>MEHKYKNHLPKIHETTFVAEGVHIIGDVEIGEDSNIWFNAVLRGDVNSIKIGRGTNIQDNATLHASTGQSPTIIGDYVTVGHNCIIHGCKIGDYSLIGMGSIILDNAEIGEYTIIGAGSLVTQNKKIPPRVLCMGSPAKVIRELTEEEIEYLKNSAKHYIELSKNYRHHHHHH[3x]

The 16S microbial community profiling of a metagenomics library from geothermal spring at Lisvori (Lesvos island, Greece) enabled the identification of a putative sequence exhibiting 95% identity to the γ‐type carbonic anhydrase (γ‐CA) from Caloramator australicus (γ‐CaCA). The sequence of γ‐CaCA was amplified by PCR, cloned, and expressed in E. coli. X‐ray crystallographic analysis of the γ‐CaCAmut structure at 2.1 Å resolution, provided detailed structural insights into how the mutations impact the overall enzyme structure, function, and thermostability. These findings provide valuable structural and functional insights into γ‐CAs and demonstrate a strategy for converting an inactive enzyme into a catalytically active form through rational design.

Activity assays showed that γ‐CaCA possesses very low, but detectable, anhydrase activity, while exhibiting no measurable esterase activity. Differential scanning fluorimetry (DSF) revealed that the enzyme shows high thermal stability with a melting temperature (T m ) approximately 65–75°C in the pH range between 5.5 and 9.0. The structure of γ‐CaCA was determined by X‐ray crystallography at 1.11 Å resolution, the highest resolution reported so far for a γ‐CA. The enzyme was crystallized as a trimer in the crystallographic asymmetric unit and contains three zinc‐binding sites, one at each interface of neighboring subunits of the trimer.(3aS,7aR)-7a-[3-(pyrimidin-5-yl)phenyl]-3a,6,7,7a-tetrahydro-4H-pyrano[4,3-d][1,3]oxazol-2-amine | C16 H16 N4 O2 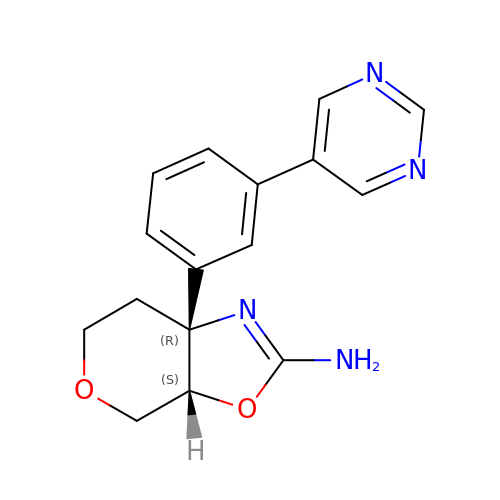| QBOAOWFKBWILHE-GDBMZVCRSA-N>GMNPAAEAEFNILLATDSYKVTHYKQYPPNTSKVYSYFECREKKTENSKLRKVKYEETVFYGLQYILNKYLKGKVVTKEKIQEAKDVYKEHFQDDVFNEKGWNYILEKYDGHLPIEIKAVPEGFVIPRGNVLFTVENTDPECYWLTNWIETILVQSWYPITVATNSREQKKILAKYLLETSGNLDGLEYKLHDFGYRGVSSQETAGIGASAHLVNFKGTDTVAGLALIKKYYGTKDPVPGYSVPAAEHSTITAWGKDHEKDAFEHIVTQFSSVPVSVVSDSYDIYNACEKIWGEDLRHLIVSRSTQAPLIIRPDSGNPLDTVLKVLEILGKKFPVTENSKGYKLLPPY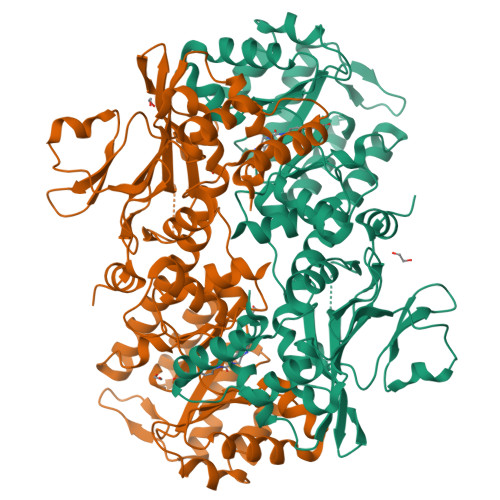LRVIQGDGVDINTLQEIVEGMKQKMWSIENIAFGSGGGLLQKLTRDLLNCSFKCSYVVTNGLGINVFKDPVADPNKRSKKGRLSLHRTPAGNFVTLEEGKGDLEEYGQDLLHTVFKNGKVTKSYSFDEIRKNAQLNIELEAAHH[2x]>[4x]MGENNMSSIAPHPVVHVALLPSAGMGHLTPFLRLASLLLHQHCHVTLITPQPTVSKAEEDLLSRFLSAFPQVNQLHFHLPPSDSTISTDPFFLQFASIRSSSHLLTPLLSSLTPPLSSFIYDMTLISPLLPIAESLGVPHYILFTSSATMFSFFAYFPTLAKSESFPGKLDFVEIPGVSVSSIPRSSI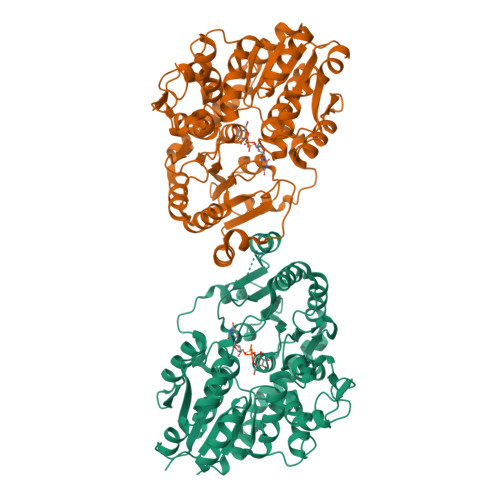PPPLLDPNSLFYKLFMEDSPKLKKLHGVLVNTFEGIEKESLEALNGGKVVKGLPPVYGVGPFVPCEFEKVVKRGETISEWLDEQPSGSVVYVSFGSRTAMGREQLREVGDGLVKSGWRFLWVVKDKIVDRAEEEGLDGVLGFELVERMVKEKKGLVVKEWVDQSEILGHKAVGGFVSHCGWNSVVEAAWFGVPILGWPLHGDQKINAEVVAKGGWGVWKEGWGWEGERLVKGEEIAEAIREVMNDESLRMKATQVKKDARKAISVGGSQEVALQKLMEVWKKNV>[4x]MAKVNAFSKKIGWIEFITGPMFAGKTAELIRRLHRLEYADVKYLVFKPKIDTRSIRNIQSRTGTSLPSVEVESAPEILNYIMSNSFNDETKVIGIDEVQFFDDRICEVANILAENGFVVIIS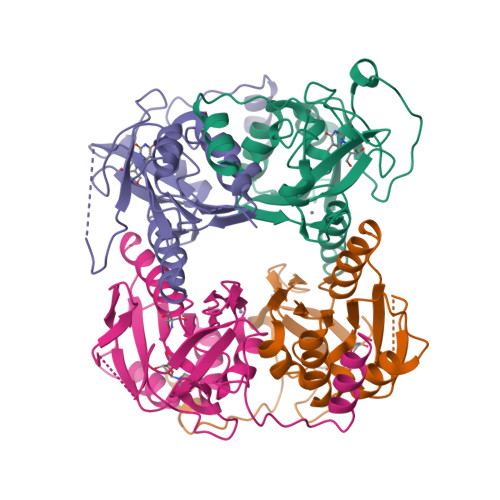GLDKNFKGEPFGPIAKLFTYADKITKLTAICNECGAEATHSLRKIDGKHADYNDDIVKIGCQEFYSAVCRHHHKVPNRPYLNSNSEEFIKFFKNKKRNKNI> MDNTPQFKPFGITYYTERVLEGATPGTTLIAVAAVDPDKGLNGLITYTLLDLTPPGYVQLEDSSAGKVIANRTVDYEEVHWLNFTVRASDNGSPPRAAEIPVYLEIVDINDNNPIFDQPSYQEAVFEDIAVGTVILRVTATDADSGNFALIEYSLVDGEGKFAINPNTGDISVLSSLDREKKDHYILTALAKDNPGDVASNRRENSVQVVIRVLDVNDCRPQFSKP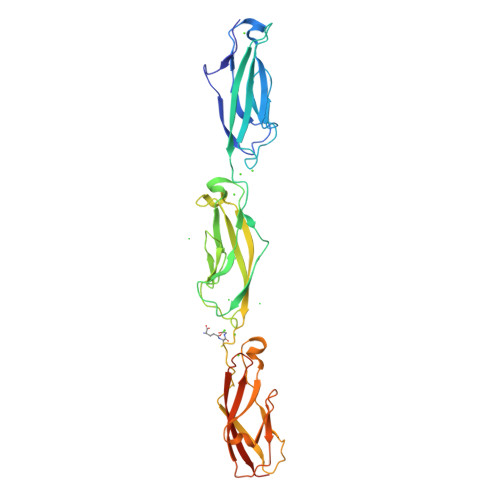QFSTSVYENEPAGTSVITMLATDQDEGSNSQLTYSLEGPGMEAFSVDMDSGLVTTQRPLQSYERFNLTVVATDGGEPPLWGTTMLLVEVIDVNDNKLAAALEHHHHHH> SMHVGIIGAGIGGTCLAHGLRKHGIKVT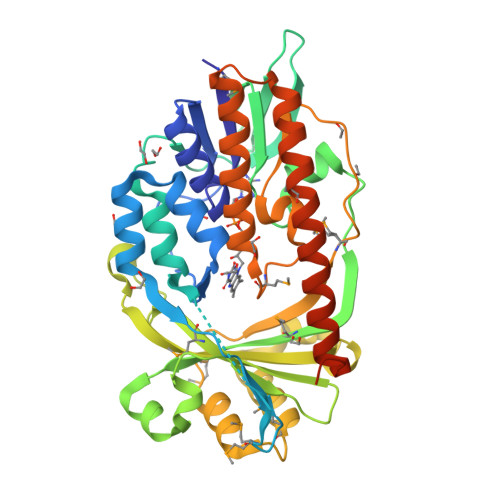IYERNSAASSILPGYGIHINSFGKQALQECLPAENWLAFEEASRYIGGQSRFYNERMRLLAVHGGISPMAGKIISEQRLSISRTELKEILNKGLANTIQWNKTFVRYEHIENGGIKIFFADGSHENVDVLVGADGSNSKVRKQYLPFIERFDVGVSMIIGRARLTPALTALLPQNFRDGTPNSIVPKSPDWLFISMWRAPVNIHVEASLAEIDNFIVWVYVAATDSLPDNITDFSAEALCDLVQSRMISWDPSLHTLVQQSDMENISPLHLRSMPHLLPWKSSTVTLLGDAIHNMTPMTGSGANTALRDALLLTQKLASVASGHEELVKAISDYEQQMRAYANEIVGISLRSAQNAVIHFSIPPLKQRHLSIRRNKSQSHQHRR>[2x]MAHHHHHHMSIKVFETREVQDLLKAASSANANGASTGDARTQQIVLRLLGDLFKAIDDLDITPDEVWAGVNYLNKLGQDGEAALLAAGLGLEKYLDIRMDAADAALGLDGGTPRTIEGPLYVAGAPVRDGVAKIDLDADAGAGPLVIHGTVKDLDGKPVAGALVECWHANSHGFYSHFDPTGAQRDFNLRGAVRTGADGTYAFRTLMPVGYGCPPQGATQQLLDRLGRHGNRPAHVH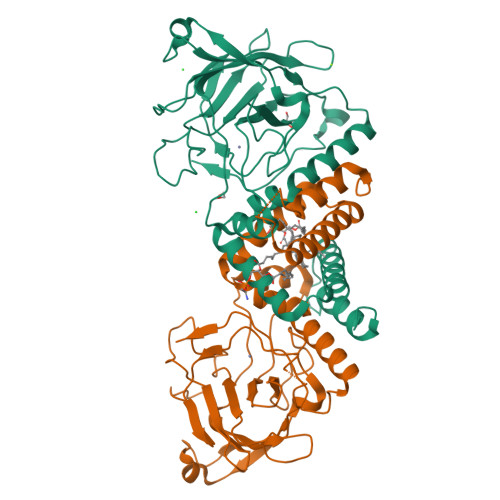FFVTSDGHRKLTTQFNIEGDPLIWDDFAYATREELIPPVTTKTGGAALGLKADAYQDITFDFVLTPRVGGADNQIVERPRASVAA>MKPLYRQLKSSHYSSDYSSPGYLAAEAVYAEIGYELDTLLKQNPGYANTCAVRMSLALLKTGISFKGRLPIKKGAYKGKTIEPGAKLLADQLHRSSSFGKAKIFFNAPDAEKGIGNKKGVVFFNKITNYDGGHIDLIEPENSLLTCHSHCYFNCK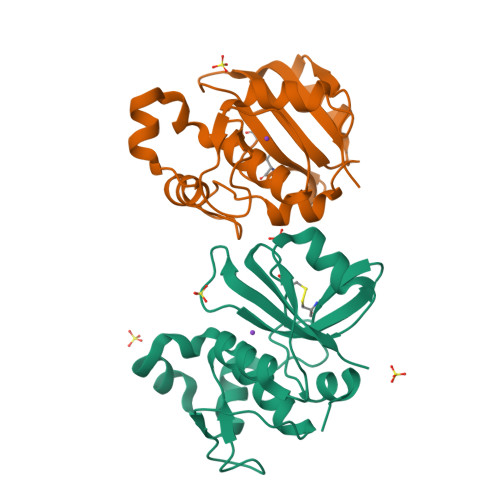EVWFWELS[2x]methyl 2-chloranyl-4-cyclohexylsulfanyl-5-sulfamoyl-benzoate 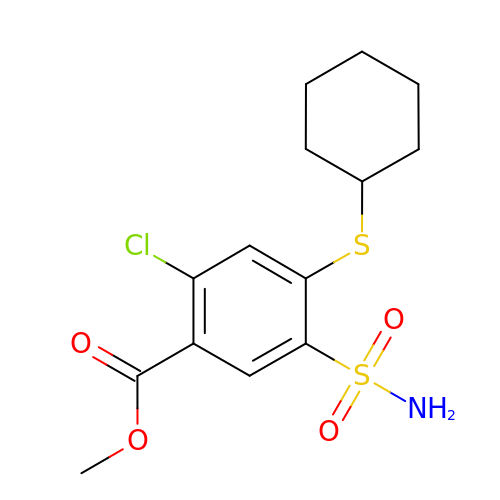| C14 H18 Cl N O4 S2 | QYEZJVLETJURBN-UHFFFAOYSA-N> MSDISFNAIPSDVRVPLTYIEFDNSNAVSGTPAPRQRVLMFGQSGSKASAAPNVPVRIRSGSQASAAFGQGSMLALMADAFLNANRVAELWCIPQGNGTGNAAVGEISLSGTAGENGSLVTYIAGQRLAVSVAAGATGAALADLLVARIKGQPDLPVTAEVRADSGDDDTHADVVLSAKFTGALSAVDVRWNYYAGETTPYGIITAFKAASGKNGNPDISASIAGMGDLQYKYIVMPYTDEPNLNLLRTELQERWGPVNQADGFAVTVLSGTYGDISTFGVSRNDHLISCMGIAGAPEPSYLYAATLCAVASQALSIDPARPLQTLTLPGRMPP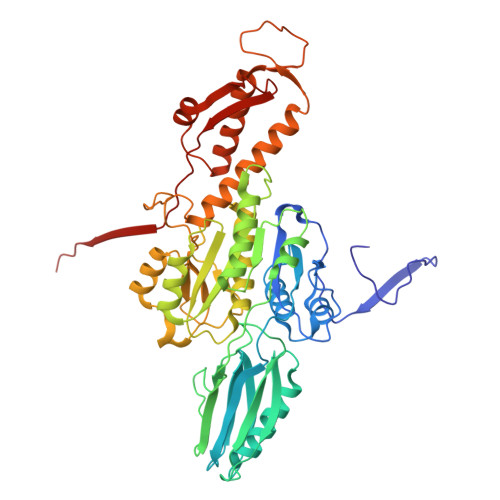AVGDRFTWSERNALLFDGISTFNVNDGGEMQIERMITMYRTNKYGDSDPSYLNVNTIATLSYLRYSLRTRITQKFPNYKLASDGTRFATGQAVVTPSVIKTELLALFEEWENAGLVEDFDTFKEELYVARNKDDKDRLDVLCGPNLINQFRIFAAQVQFIL> MNKVEPQESNAIRMIKEACEKNRRMMTDEAFRKEVE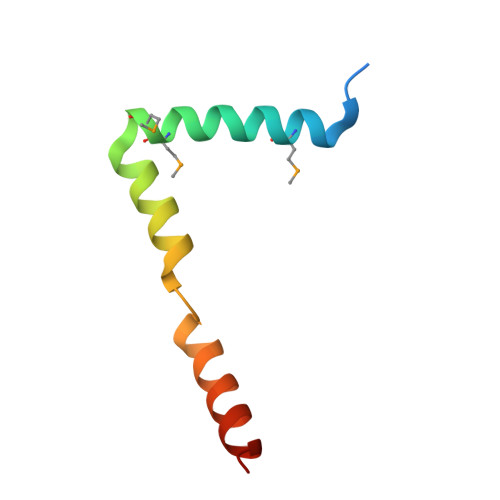KRLYAGPSPELLAKLRVLWAANKEQ(2E)-2-fluoro-3,7-dimethylocta-2,6-dien-1-yl 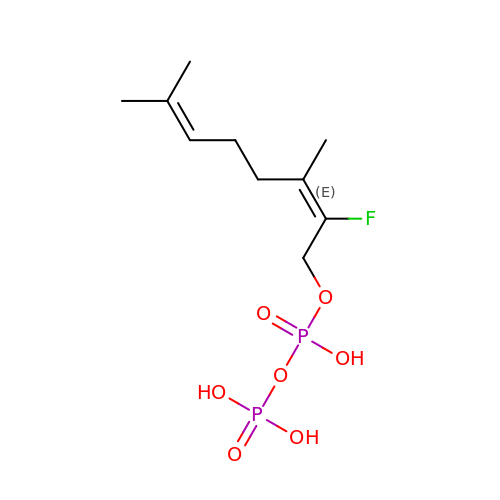trihydrogen diphosphate | C10 H19 F O7 P2 | BYJNSLXDWGDGAC-MDZDMXLPSA-N>[2x]CDKSANPKQPTQGMSVVTSFYPMYAMTKEVSGDLNDVRMIQSGAGIHSFEPSVNDVAAIYDADLFVYHSHTLEAWARDLDPNLKKSKVNVFEASKPLTLDRVKGLEDMEVTQGIDPATLYDPHTWTDPVLAGEEAVNIAKELGHLDPKHKDSYTKKAKAFKKEAEQLTEEYTQKFKKVRSK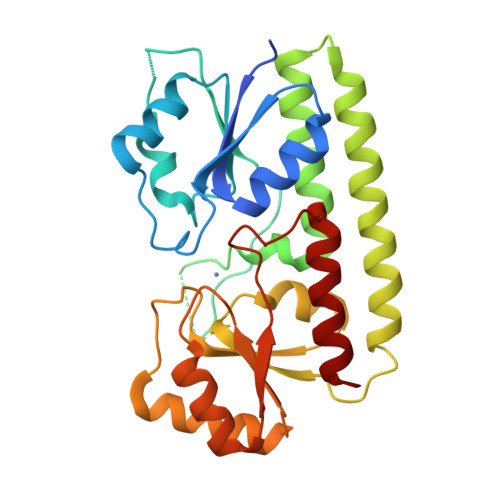TFVTQHTAFSYLAKRFGLKQLGISGISPEQEPSPRQLKEIQDFVKEYNVKTIFAEDNVNPKIAHAIAKSTGAKVKTLSPLEAAPSGNKTYLENLRANLEVLYQQLK> MSTQREYVFIPITNSITIDVKITIGGSDHITNIDERGIHNVLVITGYAVDEKNGRLVPTLDPCDYVKGILVAGTPQQAQSNDFLTLKLPANKLYLIRKKGNISDDLKIYIPYSSPDARNSMKTKPVSISDDTIVNNIIKEVFDKIYNITQKEKVKIEKVK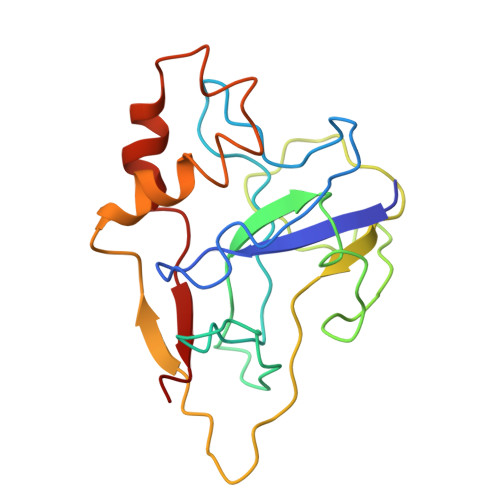EDIKELFSYYALEQ>GPGSPYGQQPQNRMMKLAYLDRGFYKHYGIIVGDHVYQLDSDDIFKTALTGKAKFTKTKLTSDWVIEEECELDYFRIKYLESAVDSEHIFSVDKNCETIAKDIFGTHTLSQHQAIGLVGTILLTAGLMSTIK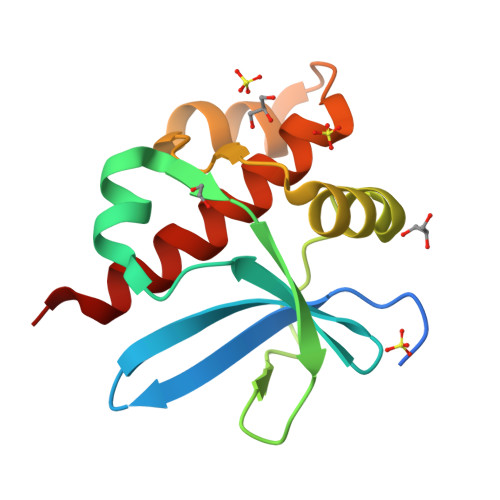[2x]>MHRTSNGSHATGGNLPDVASHYPVAYEQTLDGTVGFVIDEMTPERATASVEVTDTLRQRWGLVHGGAYCALAEMLASEATVAVVHEKGMMAVGQSNHTS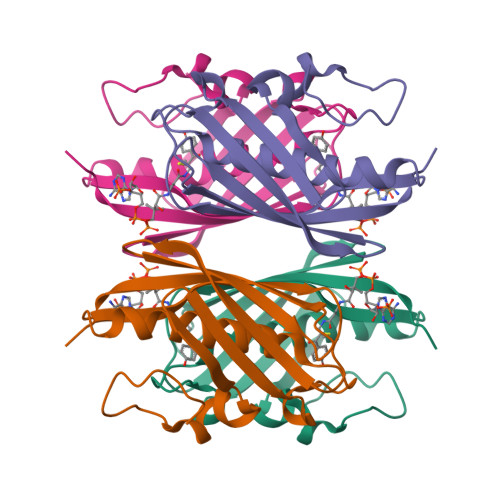FFRPVKEGHVRAEAVRIHAGSTTWFWDVSLRDDAGRLCAVSSMSIAVRPRRD[2x]> MRSTQEERFEQRIAQETAIEPQDWMPDAYRKTLIRQIGQHAHSEIVGMLPQGNWITRAPTLRRKAILLAQVQDEAGHGLYLYSAAETLGCAREDIYQKMLDGRMKYSSIFNYPTLSWADIGVIGWLVDGAAIVNQVALCRTSYGPYARAMVKICKEESFHQRQGFEACMALAQGSEAQKQMLQDAINRFWWPALMMFGPNDDNSPNSARSLTWKIKRFTNDELRQRFVDNTVPQVEMLGMTVPDPDLHFDTESGHYRFGEIDWQEFNEVINGRGICNQERLDAKRKAWEEGTWV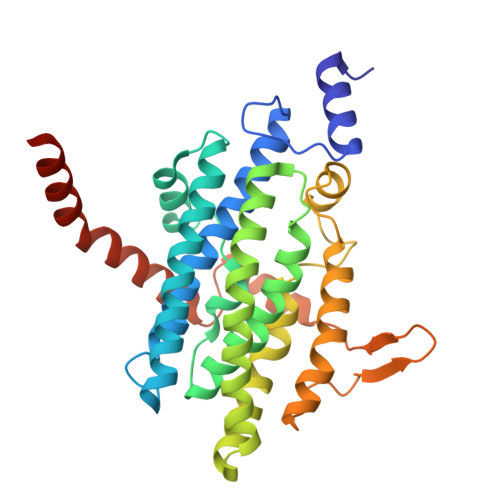REAALAHAQKQHARKVA>[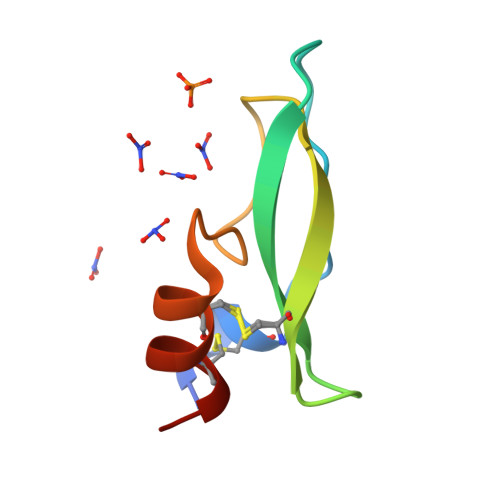2x]KDRPSLCDLPADSGSGTKAEKRIYYNSARKQCLRFDYTGQGGNENNFRRTYDCQDTCLYTA2,4-bis[(E)-(1-ethyl-3,3-dimethyl-indol-2-ylidene)methyl]cyclobutane-1,3-dione | C30 H34 N2 O2 | 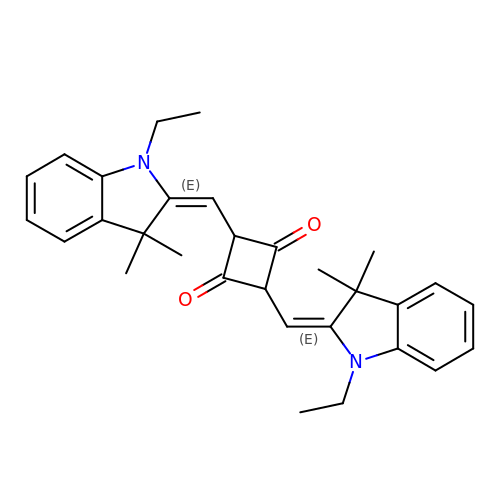RFXRJJSGFNDERY-FAKNRSBRSA-N> MESLTLQPIARVDGTINLPGSKSVSNRALLLAALAHGKTVLTNLLDSDDVRHMLNALTALGVSYTLSADRTRCEIIGNGGPLHAEGALELFLGNAGTAMRPLAAALCLGSNDIVLTGEPRMKERPIGHLVDALRLGGAKITYLEQENYPPLRLQGGFTGGNVDVDGSVSSQFLTALLMTAPLAPEDTVIRIKGDLVSKPYIDITLNLMKTFGVEIENQHYQQFVVKGGQSYQSPGTYLVEGDASSASYFLAAAAIKGGTVKVTGIGRNSMQGDIRFADVLEKMGATICWGDDYISCTRGELNAIDMDMNHIPDAAMTIATAALFAKGTTTLRNIYNWRVKETDRLFAMATELRKVGAEVEEGHDYIRITPPEKLNFAEIATYNDHRMAMCFSLVAL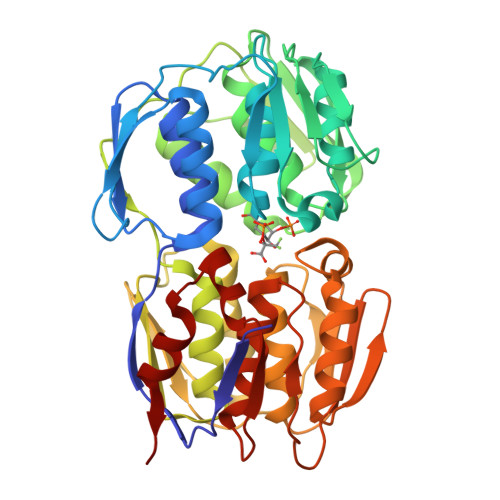SDTPVTILDPKCTAKTFPDYFEQLARISQAA> MEAAETEAEAAALEVLAEVAGILEPVGLQEEAELPAKILVEFVVDSQKKDKLLCSQLQVADFLQNILAQEDTAKGLDPLASEDTSRQKAIAAKEQWKELKATYREHVEAIKIGLTKALTQMEEAQRKRTQLREAFEQLQAKKQMAMEKRRAVQNQWQLQQEKHLQHLAEVSAEVRERKTGTQQELDRVFQKLGNLKQQAEQERDKLQRYQTFLQLLYTLQGKLLFPEAEAEAE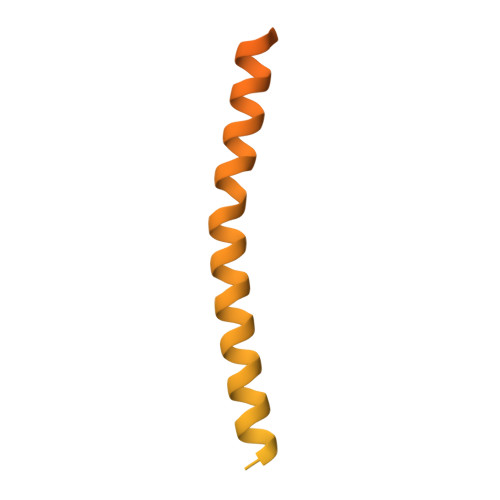NLPDDKPQQPTRPQEQSTGDTMGRDPGVSFKAVGLQPAGDVNLP> GSHMAVTGSQTALLLRAFEKDRFPGIAAREELARETGLPESRIQIWFQNRRARHP

DUX4, a member of homeobox protein family, is exclusively found in placental mammals. Compared to other homeobox proteins, DUX4 contains two adjacent HD1 and HD2 domain, connected by a short linker of 15 residues. Very recently, using next-generation sequencing technologies, a novel B-ALL oncogenic driver DUX4/IGH, derived from the insertion of chromosome fragments containing DUX4 gene into the IGH locus, has been reported in ~7% of B-ALL patients. In order to investigate how DUX4/DUX4 fusions recognize DNA, we have determined the crystal structures of Apo-DUX4HD2 and DNADRE-bound complex at the resolutions of 1.5 and 2.6 Å, respectively.

The Apo structure is a classic homeobox fold with three α-helices, termed α1, α2, α3, respectively. The N-terminal α1, α2 helices are anti-parallel. The α3 helix is perpendicular to the axis of α1/α2 helices. Compatible with its DNA binding activity, the electrostatic surface of Apo-DUX4HD2 reveals a highly positively charged pocket delineated by residues Arg137, Trp141, Arg145, Arg148, and His149 in the α3 helix.> AAGTQGAEFPELCSYTWEAVDTKNNMLYKINICGNMGVAQCGPSSAVCMHDLKTDSFHSVGDSLLKTASRSLLEFNTTVNCKQQNHKIQSSITFLCGKTLGTPEFVTATDCVHYFEWRTTAACKKNIFKANKEVPCYAFDRELKKHDLNPLIKTSGAYLVDDSDPDTSLFINVCRDIEVLRASSPQVRVCPTGAAACLVRGDRAFDVGRPQEGLKLVSNDRLVLSYVKEGAGQPDFCDGHSPAVTITFVCPSERREGTIPKLTAKSNCRFEIEWVTEYACHRDYLESRSCSLSSAQHDVAVDLQPLSRVEASDSLFYTSEADEYTYYLS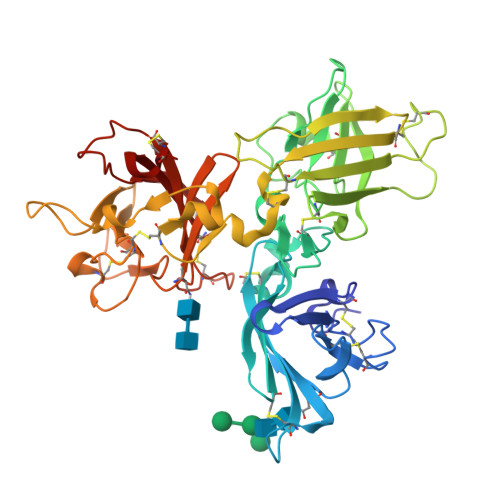ICGGSQAPICNKKDAAVCQVKKADSTQVKVAGRPQNLTLRYSDGDLTLIYFGGEECSSGFQRMSVINFECNQTAGNNGRGAPVFTGEVDCTYFFTWDTKYACV> VSITKCSSDMNGYCLHGQCIYLVDMSQNYCRCEVGYTGVR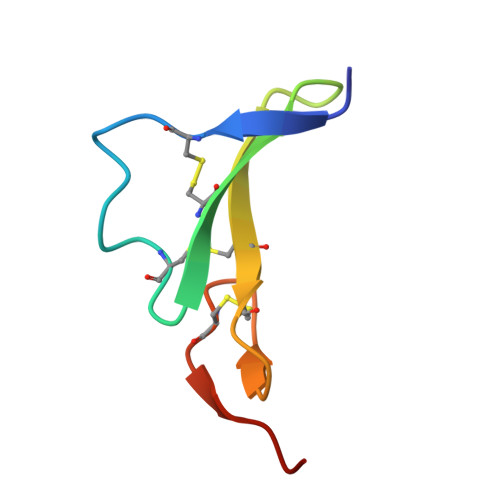CEHFFLTV> QDDSTPDSLFAGLVGEYYGTNSQLNNISDFRALVDSKEADATFEAANISYGRGSSDVAKGTHLQEFLGSDASTLSTDPGDNTDGGIYLQGYVYLEAGTYNFKVTADDGYEITINGNPVATVDNNQSVYTVTHASFTISESGYQAIDMIWWDQGGDYVFQPTLSADGGSTYFVLDSAILSSTGET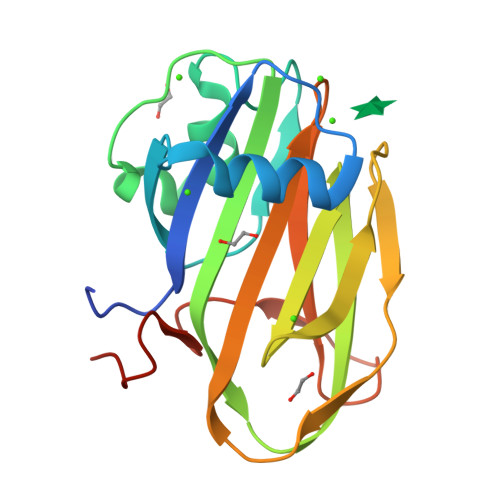PYTTAQ In plants, guanosine deaminase (GSDA) catalyzes the deamination of guanosine for nitrogen recycling and re-utilization. The other involves the hydrolysis of Gua to guanine (G), followed by its deamination to xanthine under the action of guanine deaminase (GDA). Both deaminases are zinc-dependent enzymes, which rely on a catalytic water molecule to attack the amino group-connecting C2 atom to proceed with the catalysis. The zinc ions are tightly bound to the active site, coordinated by the completely conserved residues His80, Cys113, Cys110, and the key water molecule. AtGSDA catalysis needs two key sub-processes: the activation of water and re-capping of the active site, which proceed via the two critical residues Glu82 and Tyr185, respectively.

Despite its reported strict specificity toward Gua only, we managed to identify that 2′-O-methylguanosine (2′-O-mG) and N2-methylguanosine (N2-mG) could be employed as reasonable substrates of AtGSDA by testing a series of Gua derivatives, but the structural basis is unclear. In addition, Glu82 acts as the general base to extract a proton from the catalytic water molecule, preparing the latter for the nucleophilic attack. In contrast, E82Q did not produce any products when incubated with 2′-O-mG or N2-mG under similar assay conditions. We found that while WT and Y185F/E showed similar binding affinities toward the ligands, the Y185K and E82Q mutants showed differentially reduced affinities.

>[2x]SDHKFLTQAVEEAYKGVDCGDGGPFGAVIVHNNEVVASCHNMVLKYTDPTAHAQVTAIREACKKLNKIELSECEIYASCEPCPMCFGAIHLSRLKRLVYGAKAEAAIAIGFDDFIADALRGTGVYQKSSLEIKKADGNGAAIAEQVFQNTKEKFRLY>[5x]GMENIKLGFMGLGQMGSALAH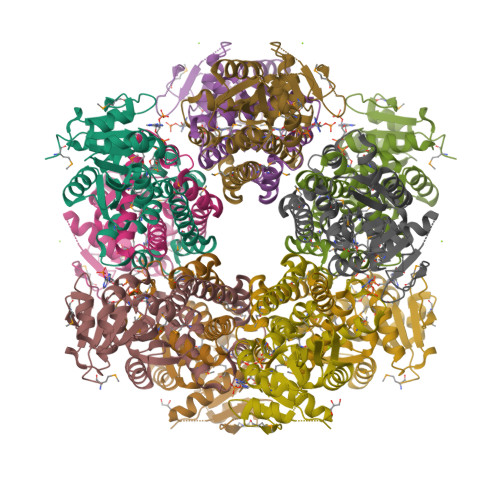GIANANIIKKENLFYYGPSKKNTTLNYMSSNEELARHCDIIVCAVKPDIAGSVLNNIKPYLSSKLLISICGGLNIGKLEEMVGSENKIVWVMPNTPCLVGEGSFIYCSNKNVNSTDKKYVNDIFNSCGIIHEIKEKDMDIATAISGCGPAYVYLFIESLIDAGVKNGLSRELSKNLVLQTIKGSVEMVKKSDQPVQQLKDNIVSPGGITAVGLYSLEKNSFKYTVMNAVEAACEKSKAMGS>MRGSHHHHHHGSMDEF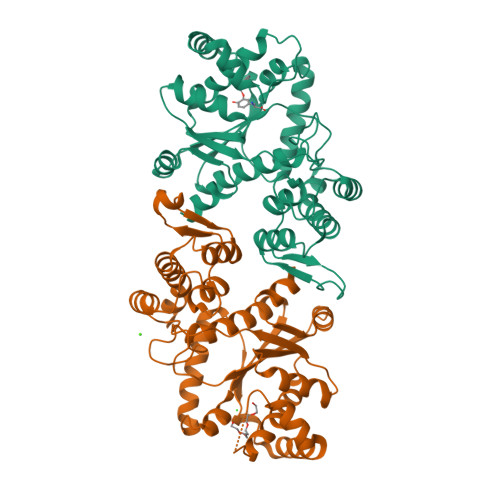EMIKRNTSEIISEEELREVLKKDEKSAAIGFEPSGKIHLGHYLQIKKMIDLQNAGFDIIIILADLAAYLNQKGELDEIRKIGDYNKKVFEAMGLKAKYVYGSEFALDKDYTLNVYRLALKTTLKRARRSMELIAREDENPKVAEVIYPIMQVNAAHYMGVDVNVGGMEQRKIHMLQRELLPKKVVCIHNPVLTGLDGEGKMSSSKGNFIAVDDSPEEIRAKIKKAYCPAGVVEGNPIMEIAKYFLEYPLTIKRPEKFGGDLTVNSYEELESLFKNKELHPMRLKNAVAEELIKILEPIRKRL[2x]C2-1-HYDROXY-2-METHYL-BUTYL-THIAMIN DIPHOSPHATE | C17 H28 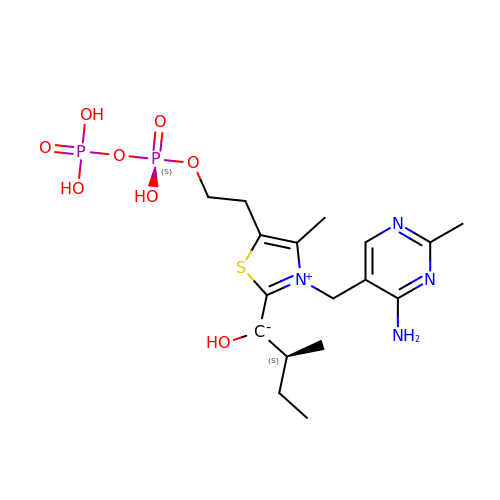N4 O8 P2 S | MZVVOGXJVCPANP-JTQLQIEISA-N methyl (2R)-2-[(4S)-6-(4-chlorophenyl)-8-methoxy-1-methyl-4H-[1,2,4]triazolo[4,3-a][1,4]benzodiazepin-4-yl]propanoate 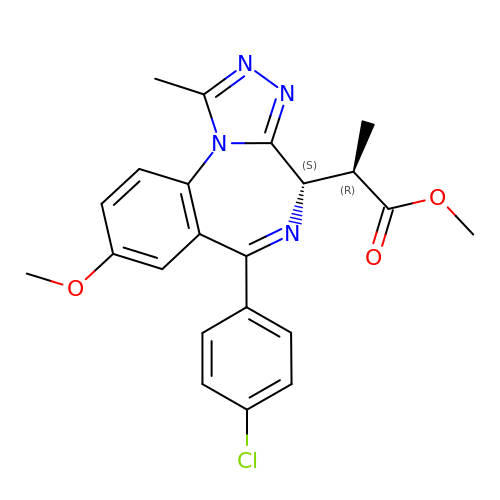| C22 H21 Cl N4 O3 | FENXDXHDXYVGRJ-BLVKFPJESA-N> PSSTMGQVGRQLAIIGDD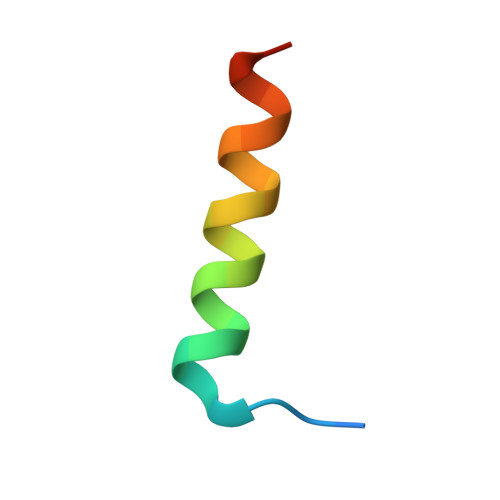INRRYDSE> NRRRRWRER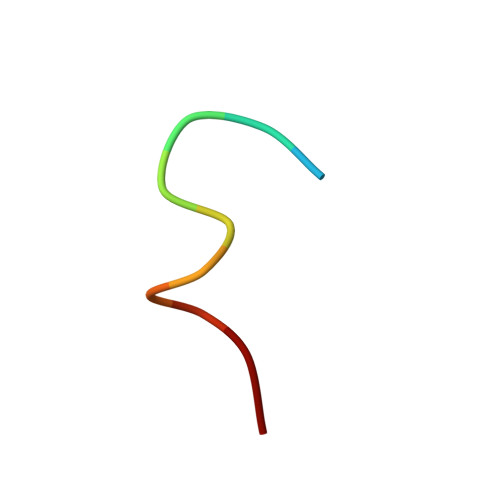QR> MAGMALARAWKQMSWFYYQYLLVTALYMLEPWERTVFNSMLVSIVGMALYTGYVFM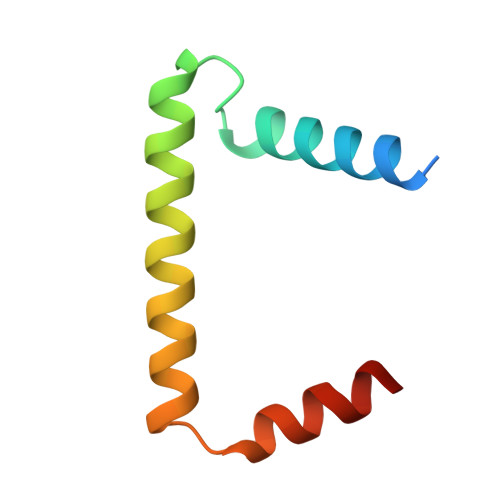PQHIMAILHYFEIVQ> MTLNQQMGITRPLKTVAKMLALASVFATSFNVFAAPVEIKFSHVVAENTPKGQMALKFKELVEQRLPGEYTVSVFPNSQLFGDNNELAALLLNDVQFVAPSLSKFERYTKRLQVFDLPFLFNDMDAVNRFQQGEAGQALLNSMSRKGIVGLGYLHNGMKQFT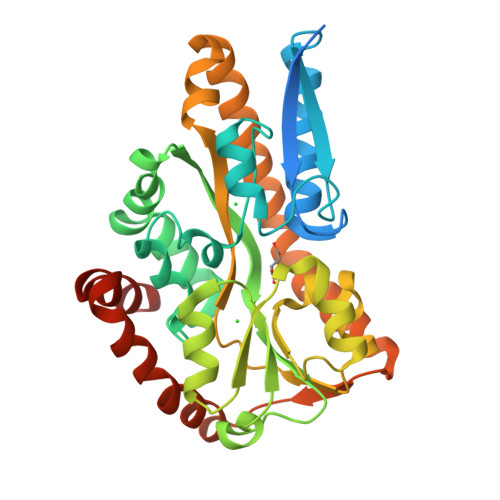ANTPLKQPSDAKGLKFRVMASDVLAAQFDAVGAIPVKKPFSEVFTLLQTRAIDGQENTWSNTYSQKFYEVQSHITESNHGVLDYMVVTSDAFWKSLPADKRKVIKEALDESIALGNKIAAEKDNEDKQLILDSKLSQLVTLSPAERQQWVDVMKPVWSKFEDQVGKDVIEAAVAANKAENLYFQ> SVGTSCIPGMAIPHN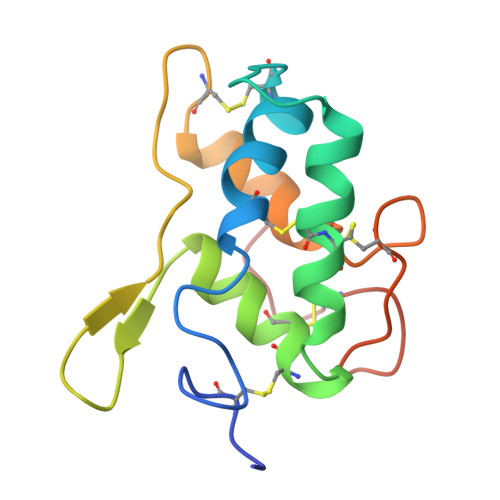PLDSCRWYVSTRTCGVGPRLATQEMKARCCRQLEAIPAYCRCEAVRILMDGVVTPSGQHEGRLLQDLPGCPRQVQRAFAPKLVTEVECNLATIHGGPFCLSLLGAGE> GPLGSMSVAGLKKQFHKATQKVSEKVGGAEGTKLDDDFKEMERKVDVTSRAVMEIMTKTIEYLAHLSSLLQAEALLA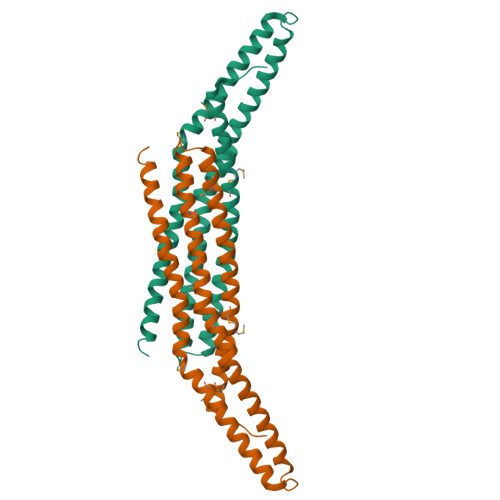EAMLKFGRELGDDCNFGPALGEVGEAMRELSEVKDSLDIEVKQNFIDPLQNLHDKDLREIQHHLKKLEGRRLDFDYKKKRQGKIPDEELRQALEKFDESKEIAESSMFNLLEMDIEQVSQLSALVQAQLEYHKQAVQILQQVTVRLEERIRQA5-azanyl-3,6-dimethyl-1H-pyrimidine-2,4-dione | C6 H9 N3 O2 | 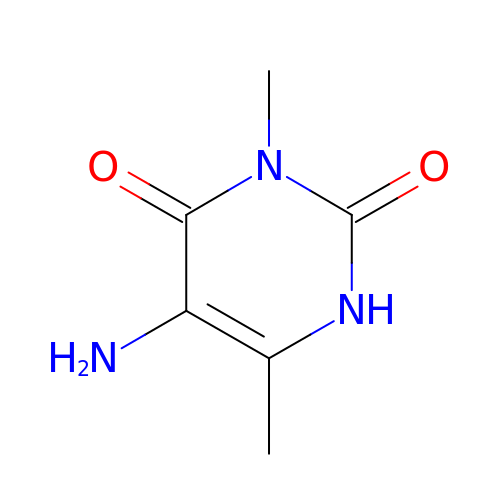DMYXWQPNMMVHBF-UHFFFAOYSA-N> MSRRAPGSRLSSGGGGGGTKYPRSWNDWQPRTDSASADPDNLKYSSSRDRGGSSSYGLQPSNSAVVSRQRHDDTRVHADIQNDEKGGYSVNGGSGENTYGRKSLGQELRVNNVTSPEFTSVQHGSRALATKDMRKSQERSMSYSDESRLSNLLRRITREDDRDRRLATVKQLKEFIQQPENKLVLVKQLDNILAAVHDVLNESSKLLQELRQEGACCLGLLCASLSYEAEKIFKWIFSKFSSSAKDEVKLLYLCATYKALETVGEKKAFSSVMQLVMTSLQSILENVDTPELLCKCVKCILLVARCYPHIFSTNFRDTVDILVGWHIDHTQKPSLTQQVSGWLQSLEPFWVADLAFSTTLLGQFLEDMEAYAEDLSHVASGESVDEDVPPPSVSLPKLAALLRVFSTVVRSIGERFSPIRGPPITEAYVTDVLYRVMRCVTAANQVFFSEAVLTAANECVGVLLGSLDPSMTIHCDMVITYGLDQLENCQTCGTDYIISVLNLLTLIVEQINTKLPSSFVEKLFIPSSKLLFLRYHKEKEVVAVAHAVYQAVLSLKNIPVLETAYKLILGEMTCALNNLLHSLQLPEACSEIKHEAFKNHVFNVDNAKFVVIFDLSALTTIGNAKNSLIGMWALSPTVFALLSKNLMIVHSDLAVHFPAIQYAVLYTLYSHCTRHDHFISSSLSSSSPSLFDGAVISTVTTATKKHFSIILNLLGILLKKDNLNQDTRKLLMTWALEAAVLMKKSETYAPLFSLPSFHKFCKGLLANTLVEDVNICLQACSSLHALSSSLPDDLLQRCVDVCRVQLVHSGTRIRQAFGK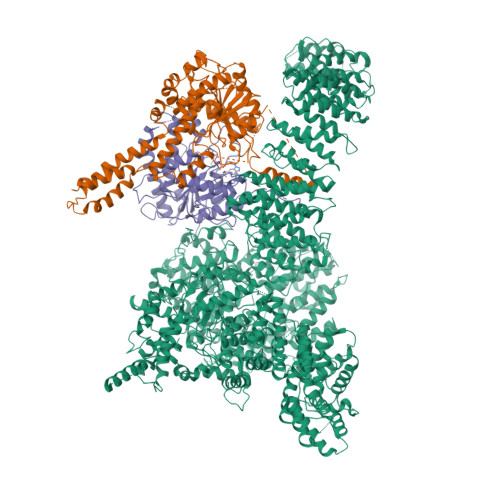LLKSIPLDVVLSNNNHTEIQEISLALRSHMSKAPSNTFHPQDFSDVISFILYGNSHRTGKDNWLERLFYSCQRLDKRDQSTIPRNLLKTDAVLWQWAIWEAAQFTVLSKLRTPLGRAQDTFQTIEGIIRSLAAHTLNPDQDVSQWTTADNDEGHGNNQLRLVLLLQYLENLEKLMYNAYEGCANALTSPPKVIRTFFYTNRQTCQDWLTRIRLSIMRVGLLAGQPAVTVRHGFDLLTEMKTTSLSQGNELEVTIMMVVEALCELHCPEAIQGIAVWSSSIVGKNLLWINSVAQQAEGRFEKASVEYQEHLCAMTGVDCCISSFDKSVLTLANAGRNSASPKHSLNGESRKTVLSKPTDSSPEVINYLGNKACECYISIADWAAVQEWQNAIHDLKKSTSSTSLNLKADFNYIKSLSSFESGKFVECTEQLELLPGENINLLAGGSKEKIDMKKLLPNMLSPDPRELQKSIEVQLLRSSVCLATALNPIEQDQKWQSITENVVKYLKQTSRIAIGPLRLSTLTVSQSLPVLSTLQLYCSSALENTVSNRLSTEDCLIPLFSEALRSCKQHDVRPWMQALRYTMYQNQLLEKIKEQTVPIRSHLMELGLTAAKFARKRGNVSLATRLLAQCSEVQLGKTTTAQDLVQHFKKLSTQGQVDEKWGPELDIEKTKLLYTAGQSTHAMEMLSSCAISFCKSVKAEYAVAKSILTLAKWIQAEWKEISGQLKQVYRAQHQQNFTGLSTLSKNILTLIELPSVNTMEEEYPRIESESTVHIGVGEPDFILGQLYHLSSVQAPEVAKSWAALASWAYRWGRKVVDNASQGEGVRLLPREKSEVQNLLPDTITEEEKERIYGILGQAVCRPAGIQDEDITLQITESEDNEEDDMVDVIWRQLISSCPWLSELDESATEGVIKVWRKVVDRIFSLYKLSCSAYFTFLKLNAGQIPLDEDDPRLHLSHRVEQSTDDMIVMATLRLLRLLVKHAGELRQYLEHGLETTPTAPWRGIIPQLFSRLNHPEVYVRQSICNLLCRVAQDSPHLILYPAIVGTISLSSESQASGNKFSTAIPTLLGNIQGEELLVSECEGGSPPASQDSNKDEPKSGLNEDQAMMQDCYSKIVDKLSSANPTMVLQVQMLVAELRRVTVLWDELWLGVLLQQHMYVLRRIQQLEDEVKRVQNNNTLRKEEKIAIMREKHTALMKPIVFALEHVRSITAAPAETPHEKWFQDNYGDAIENALEKLKTPLNPAKPGSSWIPFKEIMLSLQQRAQKRASYILRLEEISPWLAAMTNTEIALPGEVSARDTVTIHSVGGTITILPTKTKPKKLLFLGSDGKSYPYLFKGLEDLHLDERIMQFLSIVNTMFATINRQETPRFHARHYSVTPLGTRSGLIQWVDGATPLFGLYKRWQQREAALQAQKAQDSYQTPQNPGIVPRPSELYYSKIGPALKTVGLSLDVSRRDWPLHVMKAVLEELMEATPPNLLAKELWSSCTTPDEWWRVTQSYARSTAVMSMVGYIIGLGDRHLDNVLIDMTTGEVVHIDYNVCFEKGKSLRVPEKVPFRMTQNIETALGVTGVEGVFRLSCEQVLHIMRRGRETLLTLLEAFVYDPLVDWTAGGEAGFAGAVYGGGGQQAESKQSKREMEREITRSLFSSRVAEIKVNWFKNRDEMLVVLPKLDGSLDEYLSLQEQLTDVEKLQGKLLEEIEFLEGAEGVDHPSHTLQHRYSEHTQLQTQQRAVQEAIQVKLNEFEQWITHYQAAFNNLEATQLASLLQEISTQMDLGPPSYVPATAFLQNAGQAHLISQCEQLEGEVGALLQQRRSVLRGCLEQLHHYATVALQYPKAIFQKHRIEQWKTWMEELICNTTVERCQELYRKYEMQYAPQPPPTVCQFITATEMTLQRYAADINSRLIRQVERLKQEAVTVPVCEDQLKEIERCIKVFLHENGEEGSLSLASVIISALCTLTRRNLMMEGAASSAGEQLVDLTSRDGAWFLEELCSMSGNVTCLVQLLKQCHLVPQDLDIPNPMEASETVHLANGVYTSLQELNSNFRQIIFPEALRCLMKGEYTLESMLHELDGLIEQTTDGVPLQTLVESLQAYLRNAAMGLEEETHAHYIDVARLLHAQYGELIQPRNGSVDETPKMSAGQMLLVAFDGMFAQVETAFSLLVEKLNKMEIPIAWRKIDIIREARSTQVNFFDDDNHRQVLEEIFFLKRLQTIKEFFRLCGTFSKTLSGSSSLEDQNTVNGPVQIVNVKTLFRNSCFSEDQMAKPIKAFTADFVRQLLIGLPNQALGLTLCSFISALGVDIIAQVEAKDFGAESKVSVDDLCKKAVEHNIQIGKFSQLVMNRATVLASSYDTAWKKHDLVRRLETSISSCKTSLQRVQLHIAMFQWQHEDLLINRPQAMSVTPPPRSAILTSMKKKLHTLSQIETSIATVQEKLAALESSIEQRLKWAGGANPALAPVLQDFEATIAERRNLVLKESQRASQVTFLCSNIIHFESLRTRTAEALNLDAALFELIKRCQQMCSFASQFNSSVSELELRLLQRVDTGLEHPIGSSEWLLSAHKQLTQDMSTQRAIQTEKEQQIETVCETIQNLVDNIKTVLTGHNRQLGDVKHLLKAMAKDEEAALADGEDVPYENSVRQFLGEYKSWQDNIQTVLFTLVQAMGQVRSQEHVEMLQEITPTLKELKTQSQSIYNNLVSFASPLVTDATNECSSPTSSATYQPSFAAAVRSNTGQKTQPDVMSQNARKLIQKNLATSADTPPSTVPGTGKSVACSPKKAVRDPKTGKAVQERNSYAVSVWKRVKAKLEGRDVDPNRRMSVAEQVDYVIKEATNLDNLAQLYEGWTAWV;> MAGPVSLRDLLMGASAWMGSESPGGSPTEGGGSAAGGPEPPWREDEICVVGIFGKTALRLNSEKFSLVNTVCDRQVFPLFRHQDPGDPGPGIRTEAGAVGEAGGAEDPGAAAGGSVRGSGAVAEGNRTEAGSQDYSLLQAYYSQESKVLYLLLTSICDNSQLLRACRALQSGEAGGGLSLPHAEAHEFWKHQEKLQCLSLLYLFSVCHILLLVHPTCSFDITYDRVFRALDGLRQKVLPLLKTAIKDCPVGKDWKLNCRPCPPRLLFLFQLNGALKVEPPRNQDPAHPDKPKKHSPKRRLQHALEDQIYRIFRKSRVLTNQSINCLFTVPANQAFVYIVPGSQEEDPVGMLLDQLRSHCTVKDPESLLVPAPLSGPRRYQVMRQHSRQQLSFHIDSSSSSSSGQLVDFTLREFLWQHVELVLSKKGFDDSVGRNPQPSHFELPTYQKWISAASKLYEVAIDGKEEDLGSPTGELTSKILSSIKVLEGFLDIDTKFSENRCQKALPMAHSAYQSNLPHNYTMTVHKNQLAQALRVYSQHARGPAFHKYAMQLHEDCYKFWSNGHQLCEERSLTDQHCVHKFHSLPKSGEKPEADRNPPVLYHNSRARSTGACNCGRKQAPRDDPFDIKAANYDFYQLLEEKCCGKLDHINFPVFEPSTPDPAPAKNESSPAPPDSDADKLKEKEPQTQGESTSLSLALSLGQSTDSLGTYPADPQAGGDNPEVHGQVEVKTEKRPNFVDRQASTVEYLPGMLHSNCPKGLLPKFSSWSLVKLGPAKSYNFHTGLDQQGFIPGTNYLMPWDIVIRTRAEDEGDLDTNSWPAPNKAIPGKRSAVVMGRGRRRDDIARAFVGFEYEDSRGRRFMCSGPDKVMKVMGSGPKESALKALNSDMPLYILSSSQGRGLKPHYAQLMRLFVVVPDAPLQIILMPQVQPGPPPCPVFYPEKQEITLPPDGLWVLRFPYAYVTERGPCFPPKENVQLMSYKVLRGVLKAVTQ;> MSESGHSQPGLYGIERRRRWKEPGSGGPQNLSGPGGRERDYIAPWERERRDASEETSTSVMQKTPIILSKPPAERSKQPPPPTAPAAPPAPAPLEKPIVLMKPREEGKGPVAVTGASTPEGTAPPPPAAPAPPKGEKEGQRPTQPVYQIQNRGMGTAAPAAMDPVVGQAKLLPPERMKHSIKLVDDQMNWCDSAIEYLLDQTDVLVVGVLGLQGTGKSMVMSLLSANTPEEDQRTYVFRAQSAEMKERGGNQTSGIDFFITQERIVFLDTQPILSPSILDHLINNDRKLPPEYNLPHTYVEMQSLQIAAFLFTVCHVVIVVQDWFTDLSLYRFLQTAEMVKPSTPSPSHESSSSSGSDEGTEYYPHLVFLQNKARREDFCPRKLRQMHLMIDQLMAHSHLRYKGTLSMLQCNVFPGLPPDFLDSEVNLFLVPFMDSEAESENPPRAGPGSSPLFSLLPGYRGHPSFQSLVSKLRSQVMSMARPQLSHTILTEKNWFHYAARIWDGVRKSSALAEYSRLLA>GSHMASMTGGQQMGRGSEFKKYLETNGIKPKQFHKKELIFNQWDPQEYCIFLYDGITKLTSISENGTIMNLQYYKGAFVIMSGFIDTETSVGYYNLEVISEQATAYVIKINELKELLSKNLTHFFYVFQTLQKQVSYSLAKFNDFSINGKLGSICGQLLILTYVYGKETPDGIKITLDNLTMQELGYSSGIAHSSAVSRIISKLKQEKVIVYKNSCFYVQNLDYLKRYAPKLDE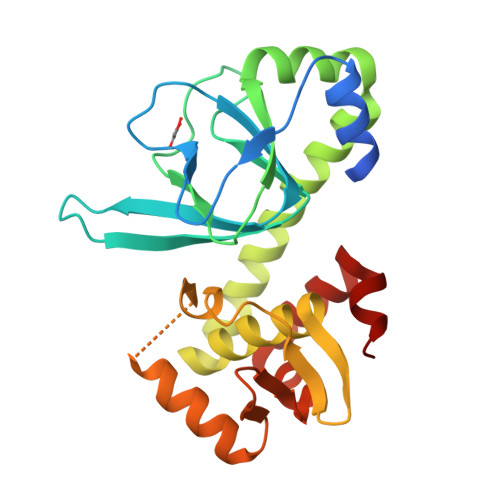WFYLACPATWGKLN[2x]>MKKVNNDTVFGILQLETLLGDINSIFSEIESEYKMSREEILILLTLWQKGSMTLKEMDRFVEVKPYKRTRTYNNLVELEWIYKERPVDDERTVIIHFNEKLQQEKVELLNFISDAI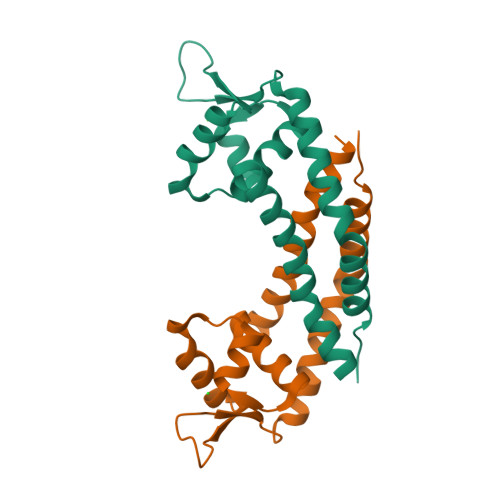ASRATAMQNSLNAIIAVHHHHHH[2x]N~1~-phenylpiperidine-1,4-dicarboxamide | C13 H17 N3 O2 | 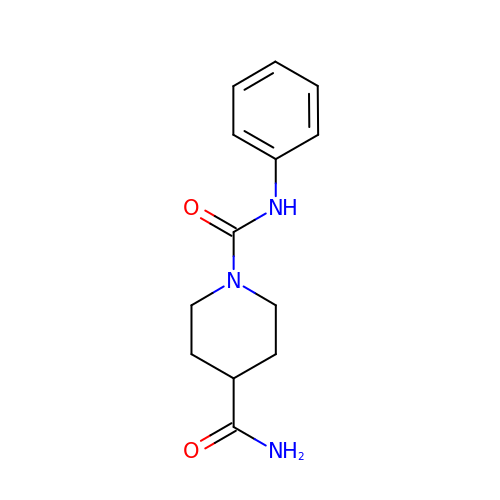OSBGPHZLIBZPGJ-UHFFFAOYSA-N>[2x]ASISGIFTTLGAAEAGDIVIRHWIDEKGIEIASERGVSAIITQDLRGKSSRLAEEHGLPVILVDRIENANALALSWTIERFAPSSRRVVVTGTNGKSTTTHMIHHIIETTGASSYTNTDSRSEFNTLIDPVVSQQIAEASSDGAPEFM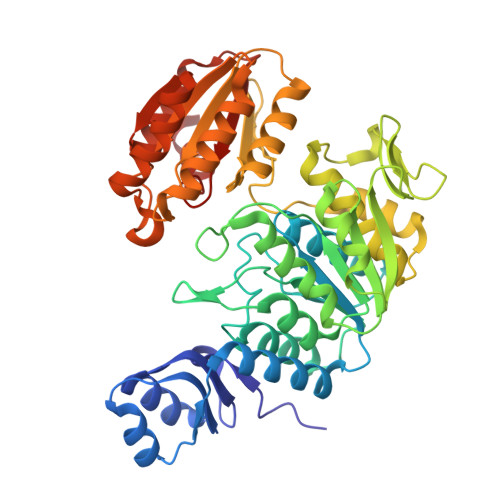VIEVSEVQGWLGRVMRDHARMMTAAIGPEVVVITNVAMDHIGLVESVEDVFREVAGALRAIESGVAVLNADDERVRAMAHVNPGLSVVFYGSDSPVRYDGEGIHIGGDLIIPAEELPFRSEHFIQNTLAAAAACLELGFSPEDIRMGVKTYRPLKRRFSVLMTEPLVIDDFAHNPSGIRFTVRSAAANLRGRLWVVNAIRGSRGEDINVMNAAALADSLRGLNAELIVTSSSDVVDEQNRVLENERRAFLGVLDERGASYIHVEKLRDALRMVLDAAKPHDTILLLGAQGMDPAAGIIDEIRM>GSMTREASPGASPEHAFRFHHIGVQTSDLENSLGWYREFFGCEQNWSLEKFSD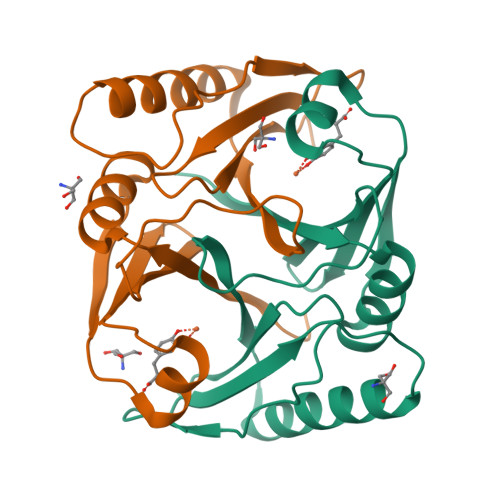LTRSRLPGITRLVELAAGDLRIHVFERAADATPAPVAEVPQFQHLCLATRSPEEMTEWRDRWLELYESGRYTFVRDEGPTDIVVDEDGVLSLYVLDVNGLEYEFTYLPEGVE[6x]> M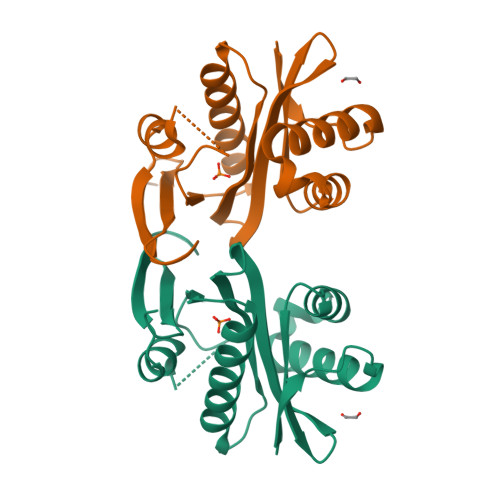IISEFDRNNPVLKDQLSDLLRLTWPEEYGDSSAEEVEEMMNPERIAVAAVDQDELVGFIGAIPQYGITGWELHPLVVESSRRKNQIGTRLVNYLEKEVASRGGITIYLGTDDLDHGTTLSQTDLYEHTFDKVASIQNLREHPYEFYEKLGYKIVGVLPNANGWDKPDIWMAKTIIPRPD4-O-methyl-beta-D-glucopyranuronic acid | C7 H12 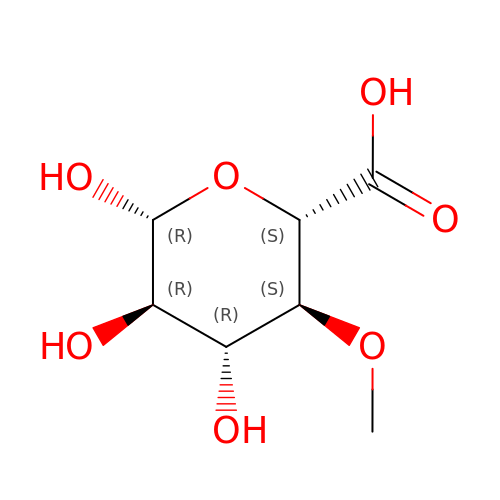O7 | WGLLPAPKWFDHHV-RLZVPWTLSA-N>VPRGSHMLYAQVNGINLHYEIEGQGQPLLLIMGLGAPAAAWDPIFVQTLTKTHQVIIYDNRGTGLSDKPDMPYSIAMFASDAVGLLDALNIPRAHVFGVSMGGMIAQELAIHYPQRVASL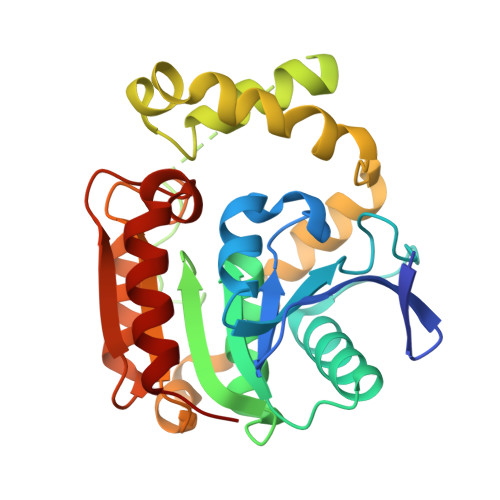ILGCTTPGGKHAVPAPPESLKALEGRAGLTPEEAIREGWKLSFSEEFIHTHKAELEAHIPRLLAQLTPRFAYERHFQATMTLRVFKQLKEIQAPTLVATGRDDMLIPAVNSEILAREIPGAELAIFESAGHGFVTSAREPFLKVLKEFLARQSV[4x]> QGVYAPAQAQIIHAGQACVVKEDNISERVYTIREGDTLVLQCLVTGHPRPQVRWTKTAGSASDKFQETSVLNETLRIEKIQRLQGGRYYCKAENGVGVPAIKSIRVDVQYLDEPVLTVHQTISDV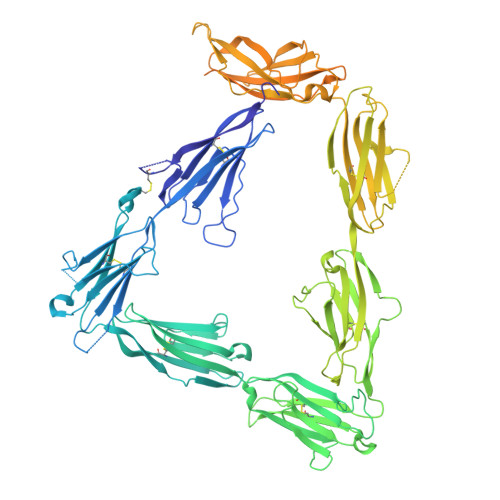RGSFYQEKTVFLRCTVNSNPPARFIWKRGAETLSHSQDNGVDIYEPLYTQGETKVLKLKNLRPQDYASYTCQVSVRNVCSIPDKSITFQLTNTTAPPALKLSVNETLVVNPGDNVTMQCSLTGGDPQPEVLWSHSPGPLPPNSLVQGGNLTIWRIRVEDSGYYNCTAINNVGNPAKKTVNLLVRSMKNATFQITPDVIKESETIQLGQDLKLSCHVDAVPQEKVVYSWYKNGKPARFSDRLLITRNDPELPPVTCSLEIIDLRFSDYGTYLCVATFQGAPIPDLSVEVNISSETVPPTISVPKGQSTITVREGSRAELQCEVRGKPKPPIIWSRVDKETPMPSGTMTVETYDGKLRLESVSRDMSGTYKCQTARYNGFNIRPREALVQLNVQFPPVVEPAFQDVRQGMGRSVTLRCTMLKGSPMKVATSVWRFNGTLLAQPPAEQQDYSELKVDSVSRETSGSYECSISNDVGVSACLFQVSAKAYSPEFYYDTPNPTLSQKQSKNYSYILQWTQKEPDAVDPILKYRLEVRQLAQRNTIQTFIPVQKMEKGLLLEHILPNLKVPQSYEVRLTPITSFGAGDMAARIIRYMEPINYPSPTDNTCRFEDEKICGFVQDKMDNFDWTRQNALTQNPKRTVNTGPPTDISGTPEGYYMFIEASRPRVTGDKARLISPLYNITAKYYCVSFYYHMYGKHIGSLNLLVRVRNKRAIDTQVWSLSGNRGNMWQQAHVPINPPGPFQIIFEGVRGTSYEGDIAIDDVTLKKGDCPRKPIGPNKGTKHHHHHH> MQWQTKLPLIAILRGITPDEALAHVGAVIDAGFDAVEIPLNSPQWEQSIPAIVDAYGDKALIGAGTVLKPEQVDALARMGCQLIVTPNIHSEVIRRAVGYGMTVCPGCATATEAFTALEAGAQALKIFP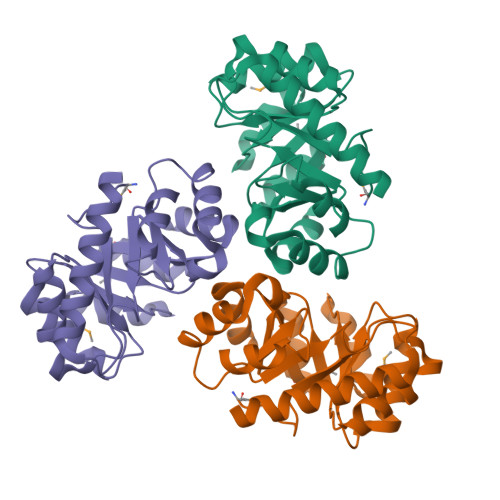SSAFGPQYIKALKAVLPSDIAVFAVGGVTPENLAQWIDAGCAGAGLGSDLYRAGQSVERTAQQAAAFVKAYREAVQLHHHHHH>MVKVDLESKRYGEKLKEVFLMLDNNVVECIKEITESSRNGKLVFFVGAGVSTLSDYPQWWRLVDKYHEELYGSPKKGNYSSDEYLRIPQIFYNVKGEMAFDGILKDFFQVDKPTNPIHDKILAMNPAHVITTNYDNLIDTACWKRGKYFSVISAEEDVANATSSRYLLKVAGDFRKGFKGENVVLKEDDYLNYDQNYPLISNLMKTIIATHTIVFIGYGLGDYNINMLLNWVRKLQKDSFHKPFFIRTDPSPIENETLIYYENKGLRIIDAASLIDSNEYDYLERYSAVMDLLIESQENKFITKDDEVIDYIYGKISPLFALQYIRKIDLKHVFEYDYHFEVNGTVVRHKNKGFGYMERFFELKESCDERSKLSKKQYERFNALFNFFEKNGVICMAKDAGTLNTSIEINSLAYHGKYDVMKKFIEEQSVSIEDDYKKAFFLACLGRWEESYDLYSNIILNSIDESNGCVYYLSQINRYRIYQSITQAVTQFNGLGLLTFGRHYKPFTDEFLARIEREMTNFNIDDLFNGMPFEFQKKYKILEFLSDNQFLYDDTVKLFELTNKVRSEMSEGSYSFGMSSDIVVLLRLYDNLRFLYENCLWSVSFHEFHQYIRNSMSLLIEKAEYERTRDIDELGFSFFGKKSGFFMEYYDFVNISRHFKIDDIKNLERSCSIDKIRFGEQEKIEEYLVGIAEEITKQFSANGMNVVFYTQFISEAKAALYFAKYVKLSEEGLGKIVKALLFYFPERDLDIGKRYVWLERLTKCNELPKSIISIIDDFLVLQAEKHIDQNYSEVSSNGLYSRDYGALIKHFEKNFISKRLSEITLCLTQDKQKQIDFLFKLLPLLSTNAKSHLLSFKSVENINDLMNGIRIGLIDEFTPEHEELIIEYLETRKVNYIVEKEKGIQTFSSNDYMSTFGIWYFLEEINNSKMEEFIGMDDQYDFFVDPENFDYKKFIPSWLKNYNDKLLGKIAGNKHMKHHVIEVLKERVKNSNDKRYLEILMNYFI[4x];>[4x]MKTVIQDTADVYFKRKSDGKLVFTAEAQTASFSQAISEEKLRGGIGNKPLYILKSEKEINLTVKNAFFDLEWLAMTQGETIQEETKVKVFDREHGLIVDDTNKVTLKGKPVSDVTFYNKKGLTYKIAVSTDGTYTIPTAFAAAKDKLTAVYQIEKVGRRLAIKASKFSERYEVEYRTIAYNPDTEEVYSDIYIQFPNVSPSGEFEMSLENGNALAPEIKFEALADTDTDEMAVVIEASRDENTAAPVEDTTGSTQSSDLGGTTE

The recently identified bacterial Sir2 domain-containing protein, defense-associated sirtuin 2 (DSR2), recognizes the phage tail tube and depletes NAD+ to abort phage propagation, which is counteracted by the phage-encoded DSR anti-defense 1 (DSAD1), but their molecular mechanisms remain unclear. DSR2 contains an N-terminal Sir2 domain that serves as an NADase effector responsible for NAD+ hydrolysis, a C-terminal domain (CTD) that functions as a sensor for detecting invading phages (as discussed later), and a middle domain (MID) that connects the Sir2 effector and the CTD sensor. DSR2 forms a tetramer with its C-terminal sensor domains (CTDs) in two distinct conformations: CTDclosed or CTDopen. Monomeric, rather than oligomeric, tail tube proteins preferentially bind to CTDclosed and activate Sir2 for NAD+ hydrolysis.

To elucidate the structural basis for the NAD+ hydrolysis by the tube-activated DSR2, we incubated the substrate (1 mM NAD+) with DSR2H171A–tube complex, which was obtained by co-expression the catalytically inactive DSR2H171A mutant and tail tube proteins together in the same bacterial cells. We then determined the cryo-EM structure of the DSR2H171A–tube–NAD+ complex at 3.0-Å resolution, in which approximately 60% density was observed, facilitating the accurate tracing of the NAD+ substrates. Further 3D classification analysis resulted in a map containing almost all parts of DSR2 at a resolution of 3.4 Å. In addition to the presence of four distinct densities corresponding to NAD+ within the Sir2 domains, we also observed four densities corresponding to the tail tube protein bound to each CTD of tetrameric DSR2 in a DSR2: tube ratio of 4:4, which is distinct from the 4:2 ratio observed for the DSR2-tube complex, indicating variability in tube binding ratio. We observed large conformational changes in the CTD by superimposing the DSR2–tube complex and the DSR2H171A–tube-NAD+ complex, likely due to their different tube binding ratios. In our determined tube-bound DSR2 structures, we observed that DSR2 interacts with phage tail tube protein in a ratio of either 4:2 in the DSR2–tube complex or 4:4 in the DSR2H171A–tube–NAD+ complex. We speculated that this variation in binding ratio can be attributed to the different purification methods we used. Given that co-expression of wild-type DSR2 with the tail tube proteins was toxic to bacterial cells, we separately expressed wild-type DSR2 and the tube proteins, and then mixed the cell pellets for the subsequent ultrasonication to obtain DSR2–tube complex, while we co-expressed DSR2H171A with the tube protein together in the same bacterial cells. Considering the tendency of the tube proteins to oligomerize once translated, the resulting lower yield of the monomeric tube proteins might have been insufficient to achieve a 4:4 binding ratio with DSR2.>[4x]MSMLTIGGKSFQSRLLLGTGKYPSFDIQKEAVAVSESDILTFAVRRMNIFEASQPNFLEQLDLSKYTLLPNTAGASTAEEAVRIARLAKASGLCDMIKVEVIGCSRSLLPDPVETLKASEQLLEEGFIVLPYTSDDVVLARKLEELGVHAIMPGASPIGSGQGILNPLNLSFIIEQAKVPVIVDAGIGSPKDAAYAMELGADGVLLNTAVSGADDPVKMARAMKLAVEAGRLSYE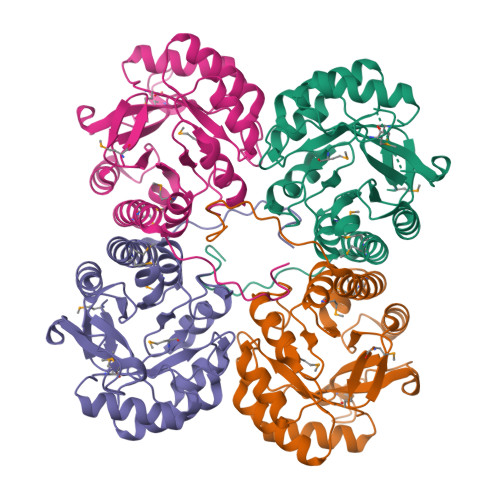AGRIPLKQYGTASSPGEGLPVLEHHHHHH>[4x]SHEELNDQLRVRREKLKKIEELGVDPFGKRFERTHK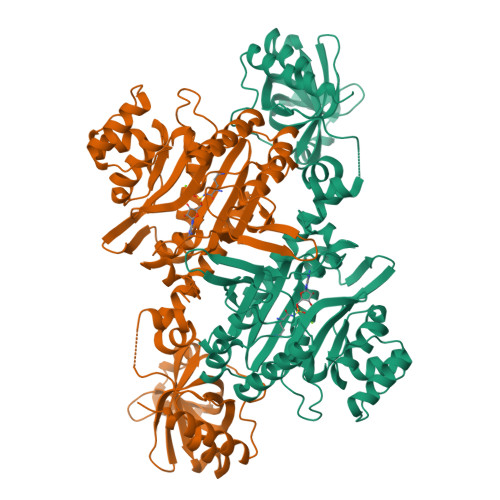AEELFELYGDLSKEELEEQQIEVAVAGRIMTKRGMGKAGFAHIQDVTGQIQIYVRQDDVGEQQYELFKISDLGDIVGVRGTMFKTKVGELSIKVSSYEFLTKALRPLPEKYHGLKDIEQRYRQRYLDLIMNPESKKTFITRSLIIQSMRRYLDSHGYLEVETPMMHAVAGGAAARPFITHHNALDMTLYMRIAIELHLKRLIVGGLEKVYEIGRVFRNEGISTRHNPEFTMLELYEAYADFRDIMKLTENLIAHIATEVLGTTKIQYGEHLVDLTPEWRRLHMVDAIKEYVGVDFWRQMSDEEARELAKEHGVEVAPHMTFGHIVNEFFEQKVEDKLIQPTFIYGHPVEISPLAKKNPDDPRFTDRFELFIVGREHANAFTELNDPIDQRQRFEEQLKEREQGNDEAHEMDEDFLEALEYGMPPTGGLGIGVDRLVMLLTNSPSIRDVLLFPQMRHK> ASAKADKKKAKEAAKAAKKKNKRAIRNSAKEADYFGDADKATTIDEQVGLIVDSLNDEELVSTADKIKANAAGAKEVLKESAKTIVDSGKLPSSLLSYFV

Ribosome associated complex (RAC), an obligate heterodimer of HSP40 and HSP70 (Zuo1 and Ssz1 in yeast), is conserved in eukaryotes and functions as co-chaperone for another HSP70 (Ssb1/2 in yeast) to facilitate co-translational folding of nascent polypeptides. On the other hand, low-resolution cryo-EM structures of the 80S-RAC complexes and biochemical characterization have identified the contact sites of RAC near the PTE of the ribosome, and more importantly demonstrated the separate binding of the C- and N-terminal parts of Zuo1 to the 40S and 60S subunits, respectively. Structural analyses indicate that RAC on the nascent-chain-free ribosome is in an autoinhibited conformation, and in the presence of a nascent chain at the peptide tunnel exit (PTE), RAC undergoes large-scale structural remodeling to make Zuo1 J-Domain more accessible to Ssb. Our data also suggest a role of Zuo1 in orienting Ssb-SBD proximal to the PTE for easy capture of the substrate.

Specifically, the C-terminal end of Zuo1 MD (residues S335 to A350) inserts into the major groove of ES12. This helix contains as many as six lysine residues, and based on our model, five of them (K337/341/342/344/348) are close to the phosphate backbone of ES12. Notably, there is no physical contact between the main body of Zuo1 4HB and ES12, except that K352 and R356 in the first helix of 4HB (the extension of the helical MD) are proximal to the phosphates of ES12. This specific embedding of a highly positively charged α-helix in the major groove could tightly lock the 4HB on ES12. Compared to the 4HB-free state, ES12 is seen to have a large rotation (~15°), with up to 13-Å displacement at the tip. Thus, together with previous genetic data, a conclusion is that multiple basic residues of Zuo1-CTD contribute to its binding to ES12, and the interaction between Zuo1-CTD and ES12 is required for the optimal function of RAC in vivo. Our structures show that Zuo1 4HB deforms ES12 in a specific way that would pose a tension to h44. Since the upper portion of h44 in the 4HB-bound state appears to be in the same conformation as in regular translating ribosomes, the effect of 4HB-ES12 interaction on the decoding center could be very subtle. Zuo1 could potentially affect the conformational dynamics of the DC through the terminal end of h44, to kinetically modulate the interactions of translation factors with the decoding center.>PTIFEERHLKYISQLGKGNFGSVELCRYDPLGDNTGALVAVKQLQHSGPDQQRDFQREIQILKALHSDFIVKYRGVSYGPGRQSLRLVMEYLPSGCLRDFL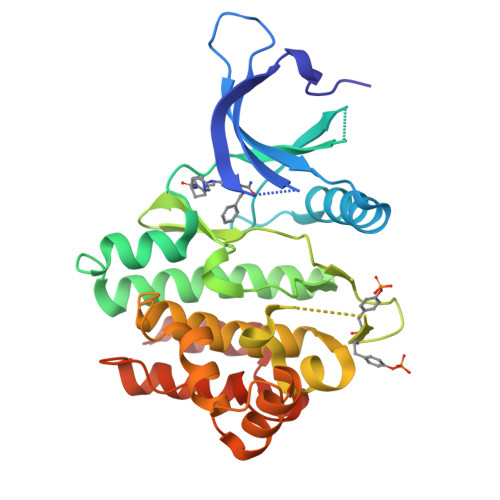QRHRARLDASRLLLYSSQICKGMEYLGSRRCVHRDLAARNILVESEAHVKIADFGLAKLLPLDKDYYVVREPGQSPIFWYAPESLSDNIFSRQSDVWSFGVVLYELFTYCDKSCSPSAEFLRMMGSERDVPALSRLLELLEEGQRLPAPPACPAEVHELMKLCWAPSPQDRPSFSALGPQLDMLWS[4x]>MRVLLIHSDYIEYEVKDKALKNPE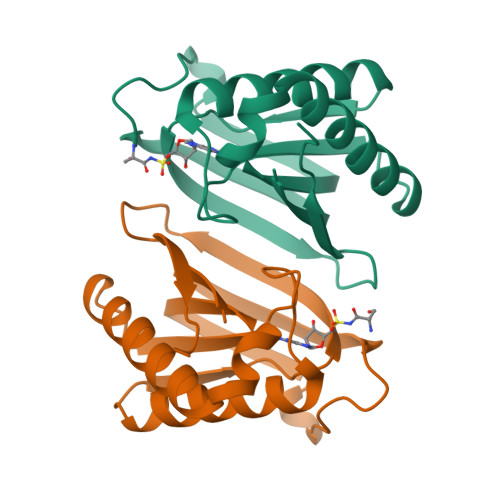PISEDMKRGRMEEVLVAFISVEKVDEKNPEEVSLKAIEEISKVAEQVKAENVFVYPFAHLSSELAKPSVAMDILNRVYQGLKERGFNVGKAPFGYYKAFKISCKGHPLAELSRTIVPEE[2x]>MIVLFVDFDYFYAQVEEVLNPSLKGKPVVVCVFSGRFEDSGAVATANYEARKFGVKAGIPIVEAKKILPNAVYLPMRKEVYQQVSSRIMNLLREYSEKIEIASIDEAYLDISDKVRDYREAYNLGLEIKNKILEKEKITVTVGISKNKVFAKIAADMAKPNGIKVIDDEEVKRLIRELDIADVPGIGNITAEKLKKLGINKLVDTLSIEFDKLKGMIGEAKAKYLISLARDEYNEPIRTRVRKSIGRIVTMKRNSRNLEEIKPYLFRAIEESYYKLDKRIPKAIHVVAVTEDLDIVSRGRTFPHGISKETAYSESVKLLQKILEEDERKIR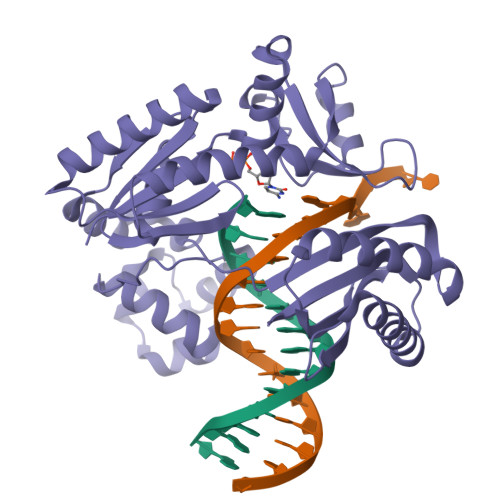RIGVRFSKFIEAIGLDKFFDT[4x]>ADKEL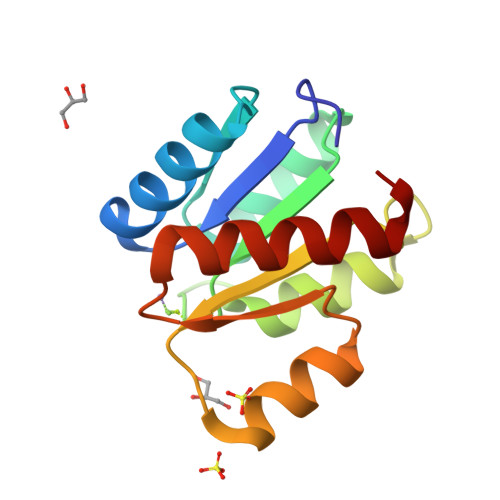KFLVVDDESTMRRIVRNLLKELGFNNVEEAEDGVDALNKLQAGGYGFVISDWMMPNMDGLELLKTIRADGAMSALPVLMVTALAKKENIIAAAQAGASGYVVKPFTAATLEEKLNKIFEKLGM[2x]>MEREKNTLPQKACHWMAAVIISLFVLPPVHAQRQTQTINDSWKFLKGECTAAADSAFDDSKWTSIHLPHTWNTDAYTEKDYYRGTGWYRRQLTLPQGWKEKQIILRLDAAGKSATIYINGKNVGEHAGGYTACSFNITPFLSFDTPNTLAVCVDNARQDIAPISGDFTFFGGIYRDVWLTAVPNQHFNLTNHGSDGLFISTPQVSEEQATLSIRGEVKNDAPEKATLELTHTIYRPDGTLLQTLKKNIQLKAGETYAFSNEATPVLKPELWTPETPRLYRVETTLRNRKTKTLLDQSNHYTAFRWFRFDGDEGFFLNGKPYKLRGICRHQDQKPIGPALTAEMHRRDFLLMKEMGANFIRISHYPQADALLEMCDKLGMLAWEEIPIIDIVPNTPGYGDNCERNLREMIRQHYNHPSIITWGYMNEILLVTQRKYKTEAELKPVLERTLALANRLERVLKEEDSTRISTMAFHGSNSYNETGLSKITDIVGWNLYQGWYGGDLTGFEKFLAQQHQNHPTHPMIVSEYGAGSDKRLHSL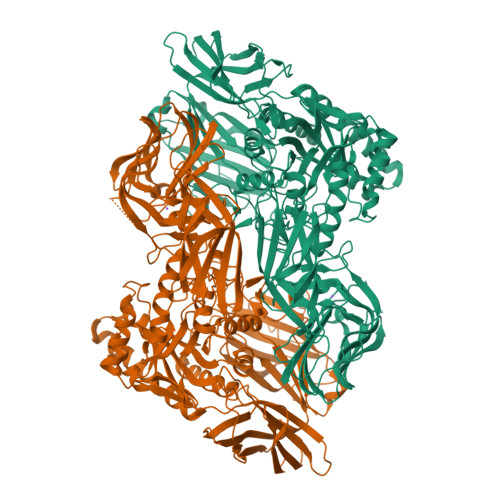HPRAFDFSIEYQQKYLEHYLPVLEDTPYICGGTHWNFIDFSSALRDESMPRINNKGLVYADRTPKDVYHYYQAAWRKDIPVLHIASRDWTDRAGVQQGNAPVYLPVKIYTNLSEVELFIDGISLGKQKTENYTATFEVPFSNRNPFLFAQGNYQGKTVQDGLRINFTPIPACLDANNLKGLELAVNVGSQCFFTSDESQLTWLPDQPYAAGSWGYIGGKEGTAQTEIQNTADGPLFQTLRNEIEGYRFDAPQGVYEIELLFTDIFRRNAGIAYQLDRNGQQENRESTFGISINGEVVEESLSPCKESGYFRALRKKYYITNDKEYIDIRFHSTSGTCFLNGIKLRNIY[2x]N-(2,6-diethylphenyl)-N'-(N-methylcarbamimidoyl)urea | C13 H20 N4 O | 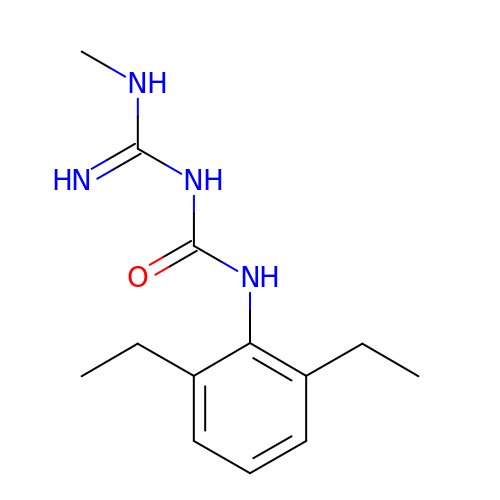IFRGRUBTWVGYDT-UHFFFAOYSA-N> MARGMNHVYLIGALARDPELRYTGNGMAVFEATVAGEDRVIGNDGRERNLPWYHRVSILGKPAEWQAERNLKGGDAVVVEGTLEYRQWEAPEGGKRSAVNVKALRMEQLGTQPELIQDAGGGVRMSGAMNEVLVLGNVTRDPEIRYTPAGDAVLSLSIAVNENYQDRQGQRQEKVHYIDATLWRDLAENMKELRKGDPVMIMGRLVNEGWTDKDGNKRNSTRVEATRVEALARGAGNANSGYAAATPAAPRTQTASSA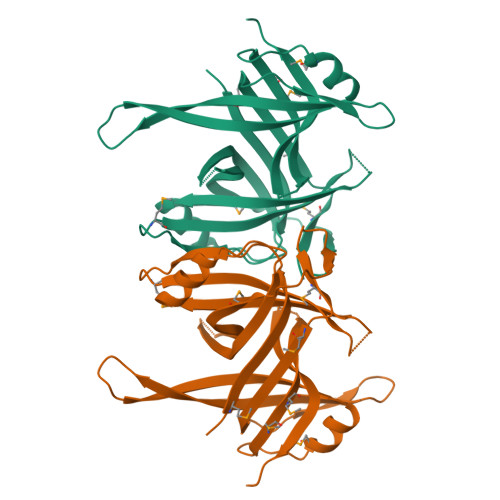ARPTSGGYQSQPSRAANTGSRSGGLDIDQGLDDFPPEEDDLPF> RAANDPFTIVHGNTGKCIKPVYGWIVADDCDETEDKLWKWVSQHRLFHLHSQKCLGLDITKSVNELRMFSCDSSAMLWWKCEHHSLYGAARYRLALKDGHGTAISNASDVWKKGGSEESLCDQPYHEIYTRDGNSYGRPCEFPFLIDGTWHHDCILDEDHSGPWCATTLNYEYDRKWGICLKPENGCEDNWEKNEQFGSCYQFNTQTALSWKEAYVSCQNQGADLLSINSAAELTYLKEKEGIAKIFWIGLNQLYSARGWEWSDHKPLNFLNWDPDRPSAPTIGGSSCARMDAESGLWQSFSCEAQLPYVCRKPLNNTVELTDVWTYSDTRCDAGWLPNNGFCYLLVNESNSWDKAHAKCKAFSSDLISIHSLADVEVVVTKLHNEDIKEEVWIGLKNINIPTLFQWSDGTEVTLTYWDENEPNVPYNKTPNCVSYLGELGQWKVQSCEEKLKYVCKRKGEKLNDASSDKMCPPDEGWKRHGETCYKIYEDEVPFGTNCNLTITSRFEQEYLNDLMKKYDKSLRKYFWTGLRDVDSCGEYNWATVGGRRRAVTFSNWNFLEPASPGGCVAMSTGKSVGKWEVKDCRSFKALSICKKMSGPLGPEEASPKPDDPCPEGWQSFPASLSCYKVFHAERIVRKRNWEEAERFCQALGAHLSSFSHVDEIKEFLHFLTDQFSGQHWLWIGLNKRSPDLQGSWQWSDRTPVSTIIMPNEFQQDYDIRDCAAVKVFHRPWRRGWHFYDDREFIYLRPFACDTKLEWVCQIPKGRTPKTPDWYNPDRAGIHGPPLIIEGSEYWFVADLHLNYEEAVLYCASNHSFLATITSFVGLKAIKNKIANISGDGQKWWIRISEWPIDDHFTYSRYPWHRFPVTFGEECLYMSAKTWLIDLGKPTDCSTKLPFICEKYNVSSLEKYSPDSAAKVQCSEQWIPFQNKCFLKIKPVSLTFSQASDTCHSYGGTLPSVLSQIEQDFITSLLPDMEATLWIGLRWTAYEKINKWTDNRELTYSNFHPLLVSGRLRIPENFFEEESRYHCALILNLQKSPFTGTWNFTSCSERHFVSLCQKYSEVKSRQTLQNASETVKYLNNLYKIIPKTLTWHSAKRECLKSNMQLVSITDPYQQAFLSVQALLHNSSLWIGLFSQDDELNFGWSDGKRLHFSRWAETNGQLEDCVVLDTDGFWKTVDCNDNQPGAICYYSGNETEKEVKPVDSVKCPSPVLNTPWIPFQNCCYNFIITKNRHMATTQDEVHTKCQKLNPKSHILSIRDEKENNFVLEQLLYFNYMASWVMLGITYRNKSLMWFDKTPLSYTHWRAGRPTIKNEKFLAGLSTDGFWDIQTFKVIEEAVYFHQHSILACKIEMVDYKEEYNTTLPQFMPYEDGIYSVIQKKVTWYEALNMCSQSGGHLASVHNQNGQLFLEDIVKRDGFPLWVGLSSHDGSESSFEWSDGSTFDYI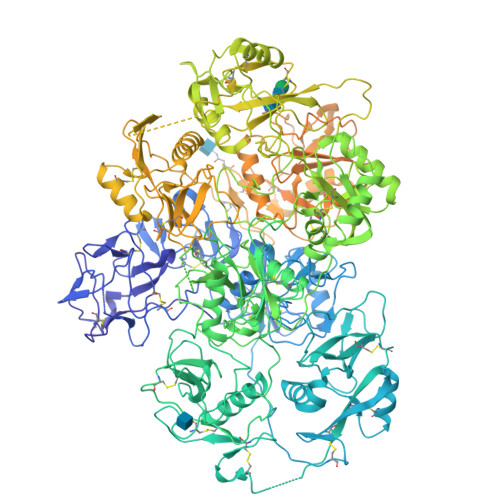PWKGQTSPGNCVLLDPKGTWKHEKCNSVKDGAICYKPTKSKKLSRLTYSSRCPAAKENGSRWIQYKGHCYKSDQALHSFSEAKKLCSKHDHSATIVSIKDEDENKFVSRLMRENNNITMRVWLGLSQHSVDQSWSWLDGSEVTFVKWENKSKSGVGRCSMLIASNETWKKVECEHGFGRVVCKVPLGPDYTAIAIIVATLSILVLMGGLIWFLFQRHRLHLAGFSSVRYAQGVNEDEIMLPSFHD>[2x]KPRQKRTATKAYNVTQAFGRRGPEQTQGNFGDQELIRQGTDYKHWPQIA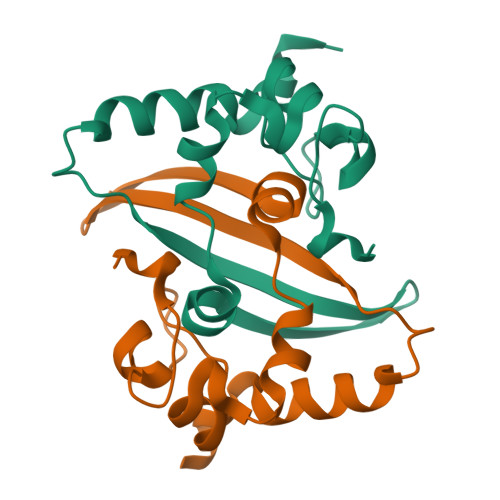QFAPSASAFFGMSRIGMEVTPSGTWLTYTGAIKLDDKDPNFKDQVILLNKHIDAYKTFP> 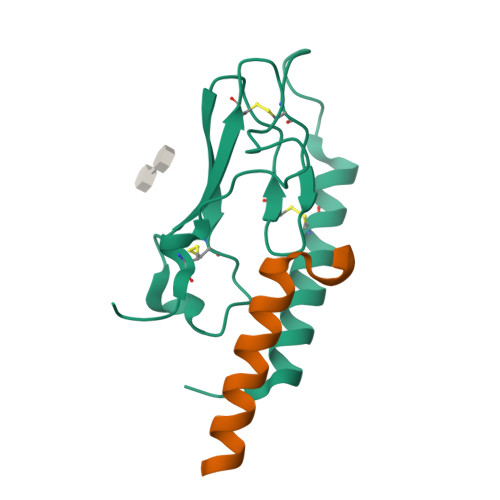RPQGATVSLWETVQKWREYRRQCQRSLTEDPPPATDLFCNRTFDEYACWPDGEPGSFVNVSCPWYLPWASSVPQGHVYRFCTAEGLWLQKDNSSLPWRDLSECEESKRGERSSPEEQLLFLY;> DLSKQMEEEAVRLFIEWLKNGGPSSGAPPPS>[4x]MKILKLQTLRGPNYWSIHRHKLVVMRLDLEDLYEKYTSDIPGFYKGLTEVLPSLVEHLCSPGVKGGFLTRVEKGTLIGHVIEHVAIELQELAGMPVGFGRTRETSTTGVFQVVIEYENEQAGRYAARAAVRLCQSIVDTGTYPATELQQDLEDLKELKNQASLGPSTEAIVKEAEARGIPWTQLGARFMIQFGYGVNQKKIQATLSNQTGILGVELACDKEGTKRILKDAGVPVPRGTVARYFDELQDAIEYVGGYPIVIKPLDGNHGRGITIDVKNWQEAEEAYDLARKASKTKTVIVERYYTGKDHRVLVVNGKVVAVAERVPAHVVGNGKSTIAELIEETNRDPQRGDGHDNILTRITVDKSALDILGKQGYSIDSIPLKGKKCFLRATANLSTGGIAVDRTDEIHPENVWLLSRVAKIIGLDIAGIDVVTEDISQPLREVEGVIVEVNAAPGFRMHVAPSRGLARNVAGAVMDMLFPGSKNGRIPILSVTGTNGKTTTTRLLAHIIKQTGKVVGYTTTDGTYIGEYLAETGDNTGPQSAHLILSDPTVEVAVLETARGGILRSGLGFSSCEVGIVLNVTADHLGIGDIDTIEQLAKLKSVVAESVMPKGYAVLNAEDPLVAAMADRVKGQVAYFSMDPNNELLLRHTEAGGLAAIYENGYISILKGDWTLRIEKAVNVPITMAGKAPFMIANALAACLAVFTQGVKIEHIRKGLSTFVASVDQTPGRMNMFNMGSYHALVDYAHNPASYEALGGFVRNWPGKRIGVVGGPGDRRDEDFVSLGELAADIFDEIIIKEDDDTRGRPRGNAAELICQGVKQFLNGIKNSESKATYESILDETAAINTALDRAPIDGLVVILPESVNRAISLIEGRHVIQDIELLQDSQREPKDQEVLKSSILEHHHHHH

Cyanophycin, a nonribosomally synthesized polypeptide consisting of equimolar amounts of aspartate and arginine as the backbone and branched sidechain, respectively, was first identified in cyanobacteria in the form of opaque and light-scattering cytoplasmic granules. The biosynthesis of cyanophycin is achieved by a single enzyme named cyanophycin synthetase (CphA1) that catalyzes peptide elongation coupled with ATP hydrolysis. The discrete active sites of the G and M domains are used for extending the Asp backbone and attaching the Arg sidechain, respectively.

In the apo state, Glid adopts an open conformation and is the furthest away from Gcore. On the other hand, the sidechain position of Phe692 in the apo form inhibits ATP binding but not the interaction between Mcore and Mlid. Mlid is not well resolved in the apo- and ATPγS-bound states, suggesting the mobile nature of Mlid. In the apo and ATPγS-bound states, a large density was observed between two Glid modules and over the binding site of (β-Asp-Arg)4 (arrowhead). CphA1 is known to synthesize cyanophycin in E. coli cells; hence, cyanophycin is the most likely candidate for the molecule with increased density.> MSLKINQAIISVFIHETEDYNKIVNTIESFFSPLISNSKKNVTTAQGHYGNKIIILEYRFDRKSGEQFFKIILEKIETSELMLILTTIDSHIDGSKLYLRFDKQYLIAEHRLVLKEGDDVIKCIISFNTSLENIKEE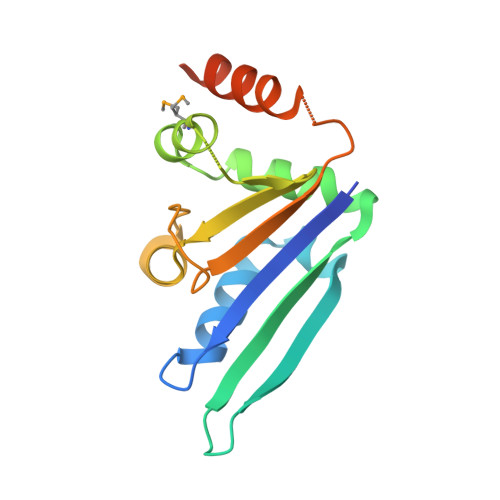IKKLVNSRIMHSKLEGHHHHHH>[2x]AK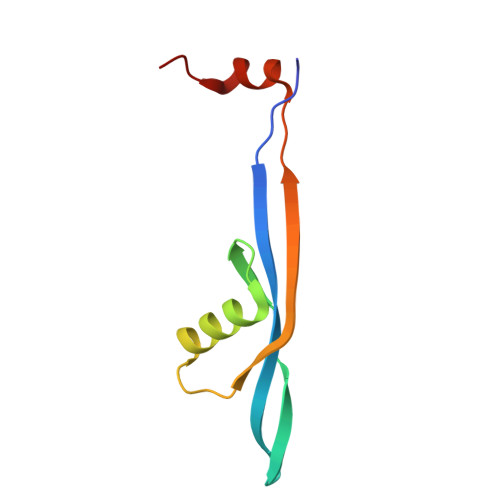MMQREITKTTVNVAKMVMVDGEVQVEQLPSETFVGNLTMEQAQWRMKRKYKGEPVQVVSVEPNTEVYELPVEKFLEVATVR>[2x]GSSMKCKFCSREAYIKIHYPKMYLCEEHFKEYFERKVSRTIERYKLLTKDERILVAVSGGKDSAVTAYVLKKLGYNIECLHINLGISGYSEKSEEYAKKQCKLIGAPLHIVRIKEILGYGIGEVKTRRPPCSYCGLTKRYIMNKFAYDNGFDAIATGHNLDDEASFLLNNILHWNTEYLAKGGPILPQQGKFIKKVKPLYEVTEREVVAYALAVGLEYIVEECPYARGA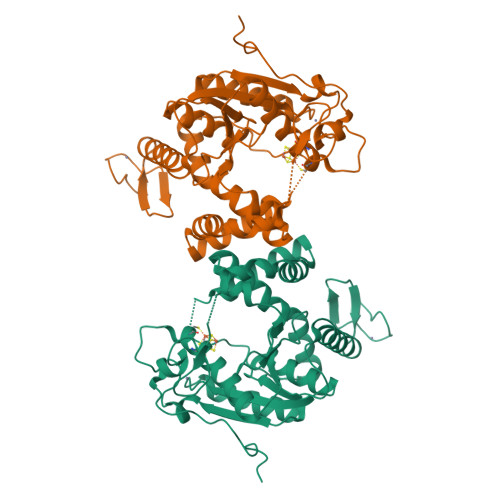TTLDMKGVLNELEEKRPGTKFNFVRGYLKKKKLFEPEIKEKEIKECKICRMPSSGDICAFCKFWGLKKEINFKVSSTDEEPFGP>MNTVVGRRIINGRRRPRRQTRRAQRPQPVVVVQTSRATQRRPRRRRRGNNRTGRTVPTRGAGSSETFVFSKDNLAGSSSGAITFGPSLSDCPAFSNGMLKAYHEYKISMVILEFVSEASSQNSGSIAYELDPHCKLNSLSSTINKFGITKPGKRAFTASYINGTEWHDVAEDQFRILYKGNGSSSIAGSFRITIKCQ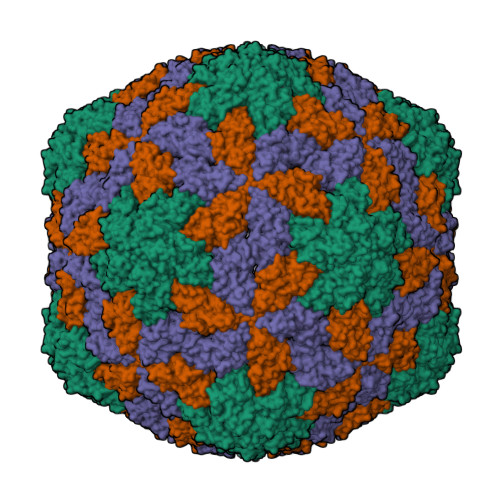FHNPK[3x]> MKTEWPELVGKSVEEAKKVILQ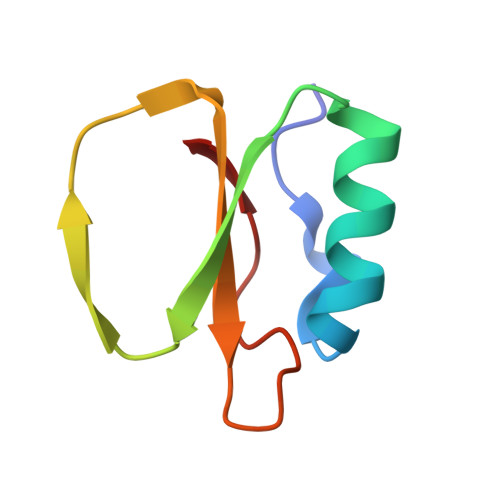DKPAAQIIVLPVGTIVTKEYRIDRVRLFVDRLDNIAQVPRVG>[4x]MSVIKPEMKIKLRMEGAVNGHKFVIEGEGIGKP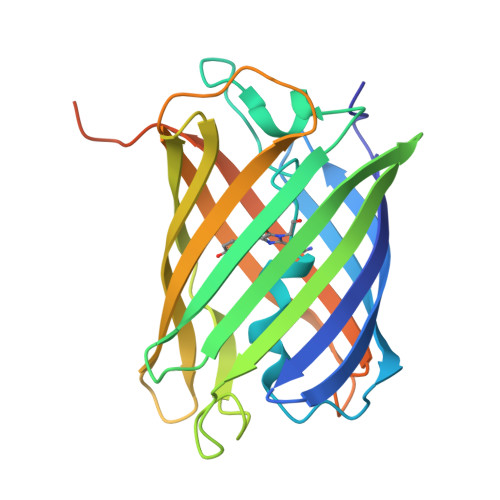YEGTQTLDLTVKEGAPLPFSYDILTPAFQYGNRAFVKYPKDIPDYFKQAFPEGYSWERSMTYEDQGICIATSDITMEGDCFFYKIRFDGTNFPPNGPVMQKKTLKWEPSTEKMYVRDGVLKGDVNMALLLEGGGHYRCDFKTTYKAKKDVRLPDAHEVDHRIEILSHDKDYNKVRLYEHAEARYSMLPSQAKASGKPIPNPLLGLDSTHHHHHH>MRALIVYTELTDKDSVISHAVARLASELNDEHVETVIIRDFEDGLAYIRSNTSIDCLLYGRDMSDRDEQIQAHRLITQLHRRQEDVPVFLLSDREEALVAFDRNMMEQVDEFAWILEDSADFIAGRVLAAIQRYRSQLLPPLMKSLIKYSDVHEYSWAAPGHQGGVGFTKTPAGRIYHDFFGENLFRTDIGIERVAVGSLLDHTGAFGECEKNAARIFGADQSYSVVVGTSGSNRTIMQACMTDDDVVVIDRNCHKSIEQGLILTGAKPVYMIPSRNRYGIIGPIYPKEMTPDAIKFKIAANPLTKGKVKQKPAYSVVTNCTYDGVCYNARKVQDLLDGSLDRIHFDEAWYGYARFNPLYRNHFAMRDEERTENEPTIFATHSTHKLLNALSQASFIHVRNGRNAIDFNRFNQAYLMHSTTSPLYAICASNDIAADMMDGNSGRSLTDEVIRESIDFRQSLAYLYKEFLNDDEWFFKPWNQEMVKDPATGKRYAFEDAPVELLMREQSCWVMHPEDKWHGFNDIPDNWAMLDPIKVSILAPGMGDDGKLLDTGVPAALVTAWLNHYGIVPTRTTDFQIMFLFSMGITKGKWGTLVNTLLSFKRHYDNNTALKKVLPEVVASAPEIYGEMGLRDLGDKMFAYLQKNNPGARLNQAYSQLPQVMMTPRDAYQQIVANRVEAVPVDQLMGRVAANSIIPYPPGIPMLLSGENFGDENSPHIHYLRSLQAWDSEFPGFEHETEGTEIIDGQYYVMCVKTCDE[20x]

Bacterial homologous lysine and arginine decarboxylases play major roles in the acid stress response, physiology, antibiotic resistance and virulence. Inducible AAT-fold basic amino acid decarboxylases (LAOdcs) have been studied since the early 1940s1,2 because of the link between their enterobacterial pathogenicity in humans and their ability to overcome the aggressive pH environments and oxygen limitation in our gastrointestinal tract. These enzymes decarboxylate either Lysine (LdcI, also called CadA), Arginine (Adc or AdiA) or Ornithine (OdcI or SpeF) into corresponding polyamines while consuming protons and producing CO2, thereby buffering the bacterial cytosol and the extracellular medium to promote bacterial survival under acid stress conditions. Here we show that the Adc from a multidrug-resistant human pathogen Providencia stuartii massively polymerises into filaments whose cryo-EM structure reveals pronounced differences between Adc and LdcI assembly mechanisms. Like all proteobacterial LAOdcs, the P. stuartii Adc monomer is organized in three different structural parts.

Moreover, as we observed P. stuartii Adc by cryo-EM with the goal to solve the structure of the decamer presented above, we discovered that most of the Adc double rings were linearly stacked to create double-rings and longer filaments. Consequently, we solved the structure of the P. stuartii Adc stacks at pH 6.5 that was used for protein purification to a resolution of 2.15 Å. The atomic model of the decamer stack reveals that upon polymerisation the conformation of the Adc decamer remains extremely similar, with minor changes localised to interfaces between monomers and dimers, and at the interface between decamers. The inter-decamer interface is mainly stabilised by a salt bridge between D472 and R492, both located in the AAT domain and respectively situated in a loop following helix α18 and in a β-hairpin. Remarkably, D472 and R492 are replaced by G472 and T492 respectively in the solved structures of E. coli and Salmonella Typhimurium Adcs, providing an explanation for the inability of these enzymes to polymerise. We note that the isoelectric point of the decamer shifts to 6 upon stacking, in line with the burial of acidic residues at the stack interface. Specifically, although the diameters of the LdcI and Adc decamers are very similar, the height of the Adc decameric ring is 105 Å compared to the 90 Å height of the LdcI decamer. This height difference, resulting in a 95 Å repeat distance between successive P. stuartii Adc stacked decamers compared to 76 Å in the LdcI stacks, is caused by an inserted β-hairpin in Adc, which contains the stack-forming residue R492, as well as by an approximately 10° rotation in the wing domain.> MTQPELTPAQRTEVELLARGRADKSRVLRDLKLPETPEAAHALLLRLGVWDEARTPYADRLRAALNAVELPVPDFDPAEERLDLTHLPTFAIDDEGNQDPDDAVGVEDLGGGLTRLWVHVADVAALVAPDSPLDLEARARGATLYLPDRTIGMLPDELVAKAGLGLHEVSPALSICLDLDPDGNAEAVDVLLTRVKVQRLAYQEAQARLEAGEEPFVTLARLARASRRLREGEGALSIDLPEVRVKADETGASVFPLPKPEMRTVVQECMTLAGWGTAIFADDNEIPLPFATQDYPTREVAGDTLPAMWARRKTLARTRFQPSPGPHH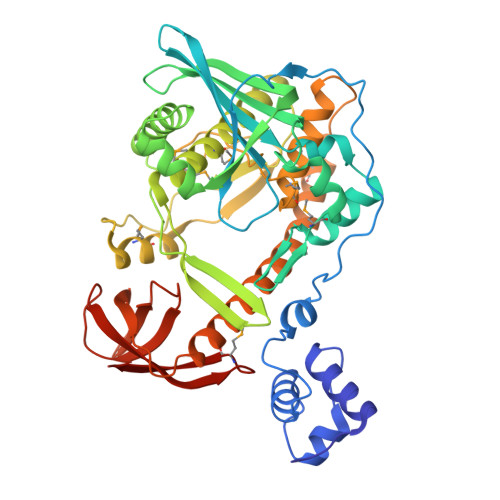GMGLDLYAQATSPMRRYLDLVVHQQLRAFLAGRDPLSSKVMAAHIAESQMNADATRQAERLSRRHHTLRFIAAQPERVWDAVVVDRRGAQATLLIPDLAFDVQVNTPAAPGTALQVQFADIDLPQMRVRARSVLEHHHHHH>QNVSLQPPPQQLIVQNKTIDLPAVYQLNGGEEANPHAVKVLKELLSGKQSSKKGMLISIGEKGDKSVRKYSRQIPDHKEGYYLSVNEKEIVLAGNDERGTYYALQTFAQLLKDGKLPEVEIKDYPSVRYRGVVEGFYGTPWSHQARLSQLKFYGKNKMNTYIYGPKDDPYHSAPNWRLPYPDKEAAQLQELVAVANENEVDFVWAIHPGQDIKWNKEDRDLLLAKFEKMYQLGVRSFAVFFDDISGEGTNPQKQAELLNYIDEKFAQVKPDINQLVMCPTEYNKSWSNPNGNYLTTLGDK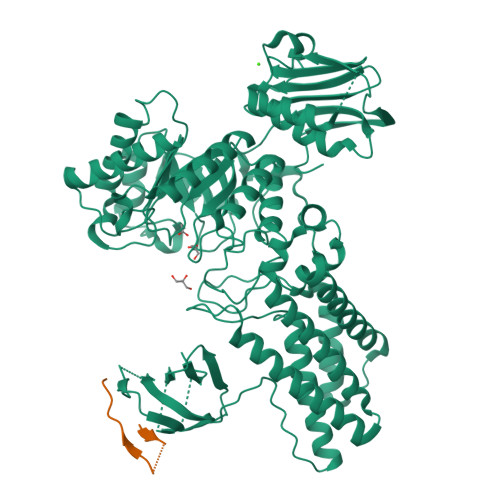LNPSIQIMWTGDRVISDITRDGISWINERIKRPAYIWWNFPVSDYVRDHLLLGPVYGNDTTIAKEMSGFVTNPMEHAESSKIAIYSVASYAWNPAKYDTWQTWKDAIRTILPSAAEELECFAMHNSDLGPNGHGYRREESMDIQPAAERFLKAFKEGKNYDKADFETLQYTFERMKESADILLMNTENKPLIVEITPWVHQFKLTAEMGEEVLKMVEGRNESYFLRKYNHVKALQQQMFYIDQTSNQNPYQPGVKTATRVIKPLIDRTFATVVKFFNQKFNAHLDATTDYMPHKMISNVEQIKNLPLQVKANRVLISPANEVVKWAAGNSVEIELDAIYPGENIQINFGKDAPCTWGRLEISTDAKEWKTVDLKQKESRLSAGLQKAPVKFVRFTNVSDEEQQVYLRQFVLTIEKK[2x]> NECLGTIGPVTPLDASDFALDIRMPGVTPKESDTYFCMSMRLPVDEEAFVIDFKPRASMDTVHHMLLFGCNMPSSTGSYWFCDEGTCTDKANILYAWARNAPPTRLPKGVGFRVGGETGSKYFVLQVHYGDISAFRDNHKDCSGVSVHLTRVPQPLIAGMYLMMSVDTVIPPGEKVVNADISCQYKMYPMHVFAYRVHTHHLGKVVSGYRVRNGQWTLIGRQNPQLPQAFYPVEHPVDVTFGDILAARCVFTGEGRTEATHIGGTSSDEMCNLYIMYYMEAKYALSFMTCTKNVAPDMFRTIPAEANI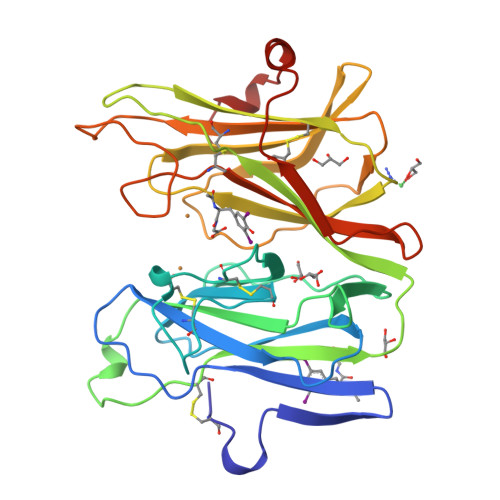PI>MANVVAEGAYPYCRLTDQPLSVDEVLAAVSGP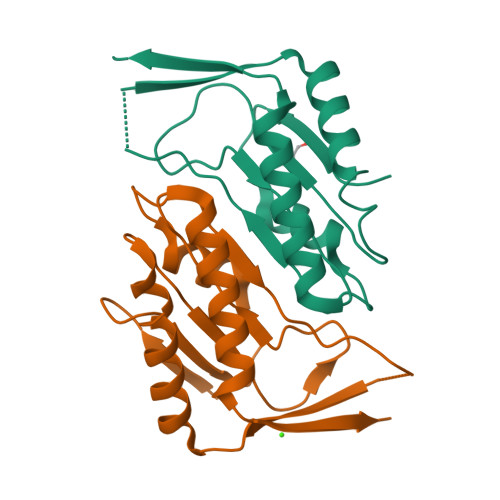EQGGIVIFVGNVRDHNAGHDVTRLFYEAYPPMVIRTLMSIIGRCEDKAEGVRVAVAHRTGELQIGDAAVVIGASAPHRAEAFDAARMCIELLKQEVPIWKKEFSSTGAEWVGDRP[2x]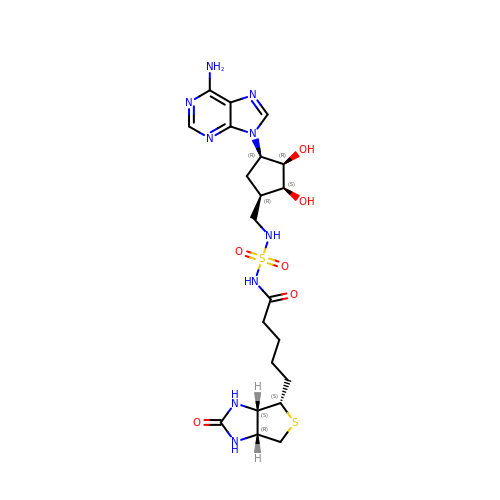N-({[(1R,2S,3R,4R)-4-(6-amino-9H-purin-9-yl)-2,3-dihydroxycyclopentyl]methyl}sulfamoyl)-5-[(3aS,4S,6aR)-2-oxohexahydro-1H-thieno[3,4-d]imidazol-4-yl]pentanamide | C21 H31 N9 O6 S2 | HTTJGHVBXHXTNE-INFCYNJXSA-N>MQFSKMHGLGNDFMVVDAVTQNVFFSPELIRRLADRHLGVGFDQLLVVE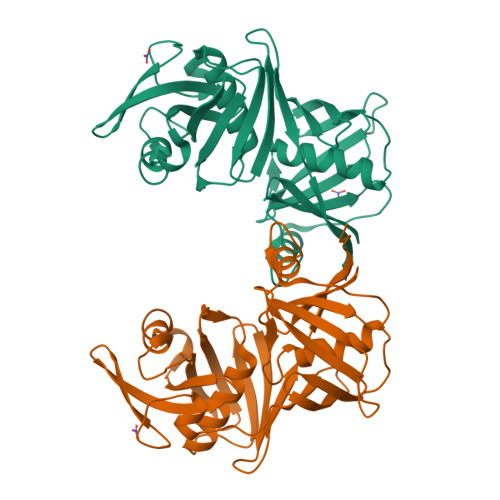PPYDPELDFHYRIFNADGSEVAQCGNGARCFARFVRLKGLTNKRDIRVSTANGRMVLTVTDDDLVRVNMGEPNFEPSAVPFRANKAEKTYIMRAAEQTILCGVVSMGNPHCVIQVDDVDTAAVETLGPVLESHERFPERANIGFMQVVKREHIRLRVYERGAGETQACGSGACAAVAVGIQQGLLAEEVRVELPGGRLDIAWKGPGHPLYMTGPAVHVYDGFIHLHHHHHH[2x]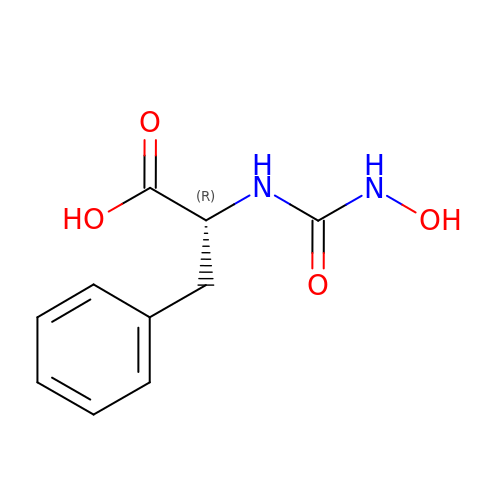D-[(N-HYDROXYAMINO)CARBONYL]PHENYLALANINE | C10 H12 N2 O4 | IOFPEOPOAMOMBE-MRVPVSSYSA-N> MHFEAYPPEVNSANIYAGPGPDSMLAAARAWRSLDVEMTAVQRSFNRTLLSLMDAWAGPVVMQLMEAA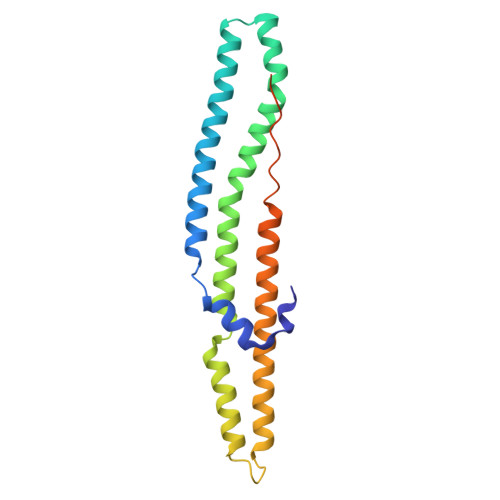KPFVRWLTDLCVQLSEVERQIHEIVRAYEWAHHDMVPLAQIYNNRAERQILIDNNLLGQFTAQIADLDQEYDDFWDEDGEVMRDYRLRVSDALSKLTPWKAPPPIAHSTVLVAPVSPSTASSRTDT>[2x]MSELFSVPYFIENLKQHIEMNQSEDKIHAMNSYYRSVVSTLVQ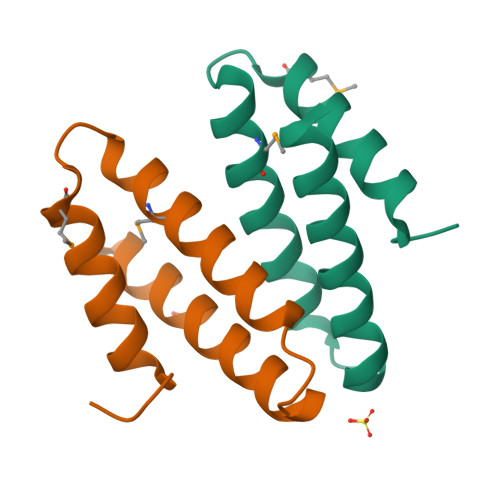DQLTKNAVVLKRIQHLDEAYNKVKRGESKLEHHHHHH> TGVENSGAGPTSFKTM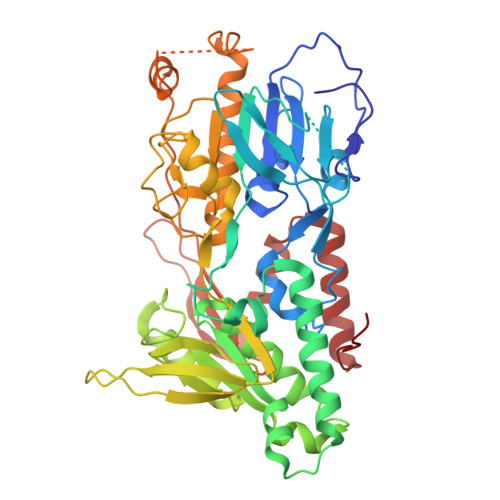KVIDPQHSDKPNVLILGSGWGAISFLKHIDTKKYNVSIISPRSYFLFTPLLPSAPVGTVDEKSIIEPIVNFALKKKGNVTYYEAEATSINPDRNTVTIKSLSAVSQLYQPENHLGLHQAEPAEIKYDYLISAVGAEPNTFGIPGVTDYGHFLKEIPNSLEIRRTFAANLEKANLLPKGDPERRRLLSIVVVGGGPTGVEAAGELQDYVHQDLRKFLPALAEEVQIHLVEALPIVLNMFEKKLSSYAQSHLENTSIKVHLRTAVAKVEEKQLLAKTKHEDGKITEETIPYGTLIWATGNKARPVITDLFKKIPEQNSSKRGLAVNDFLQVKGSNNIFAIGDNAFAGLPPTAQVAHQEAEYLAKNFDKMAQIPNFQKNLSSRKDKIDLLFEENNFKPFKYNDLGALAYLGSERAIATIRSGKRTFYTGGGLMTFYLWRILYLSMILSARSRLKVFFDWIKLAFFKRDFFKGL>[4x]MKRMLINATQQEELRVALVDGQRLYDLDIESPGHEQKKANIYKGKITRIEPSLEAAFVDYGAERHGFLPLKEIAREYFPANYSAHGRPNIKDVLREGQEVIVQIDKEERGNKGAALTTFISLAGSYLVLMPNNPRAGGISRRIEGDDRTELKEALASLELPEGMGLIVRTAGVGKSAEALQWDLSFRLKHWEAIKKAAESRPAPFLIHQESNVIVRAFRDYLRQDIGEILIDNPKVLELARQHIAALGRPDFSSKIKLYTGEIPLFSHYQIESQIESAFQREVRLPSGGSIVIDSTEALTAIDINSARATRGGDIEETAFNTNLEAADEIARQLRLRDLGGLIVIDFIDMTPVRHQRAVENRLREAVRQDRARIQISHISRFGLLEMSRQRLSPSLGESSHHVCPRCSGTGTVRDNESLSLSILRLIEEEALKENTQEVHAIVPVPIASYLLNEKRSAVNAIETRQDGVRCVIVPNDQMETPHYHVLRVRKGEETPTLSYMLPKLHEEA

RNase E is an essential bacterial endoribonuclease involved in the turnover of messenger RNA and the maturation of structured RNA precursors in Escherichia coli. The N-terminal half forms the catalytic domain (residues 1–530), resembles its paralog RNase G, and is relatively conserved among prokaryotes (Marcaida et al., 2006). The RNase E catalytic domain forms a dimer of dimers, with a quaternary organization resembling two pairs of scissors arranged in tandem. Between these two domains is a pair of conserved CPxCxGxG motifs, one on each monomer, that coordinate a single zinc ion.

Quaternary flexibility is also suggested by a second RNase E structure that we have solved to 3.5 Å and that possesses small breakdown fragments of M1 RNA. In that structure, the quaternary organization resembles the previously described holoprotein, although possessing a slight ∼10° bend, and its tertiary organization is nearly identical to that of the apoprotein. The positions of the side chains of several residues in both structures are not certain because of the poor quality of the electron density maps. Quaternary structural adjustments may occur in the binding of intricately folded RNAs, such as M1 RNA. However, the complex between the N-terminal catalytic half of RNase E and M1 RNA has one tetramer per RNA component under saturating conditions, as shown by native gel electrophoresis mobility shift assays and by nondissociating mass spectrometry (P. Ilag et al., personal communication). A bent tetramer may explain this observed 1:1 ratio of stoichiometry of tetramer to RNA.13(S)-HYDROPEROXY-9(Z),11(E)-OCTADECADIENOIC ACID | C18 H32 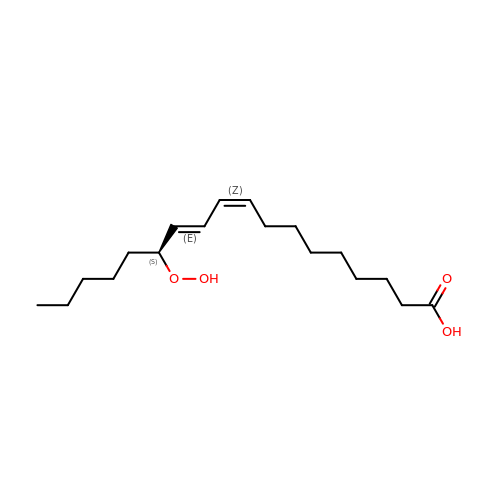O4 | JDSRHVWSAMTSSN-IRQZEAMPSA-N>GSMTISNMEADMNRLLKQREELTKRREKLSKRREKIVKENGEGDKNVANINEEMESLTANIDY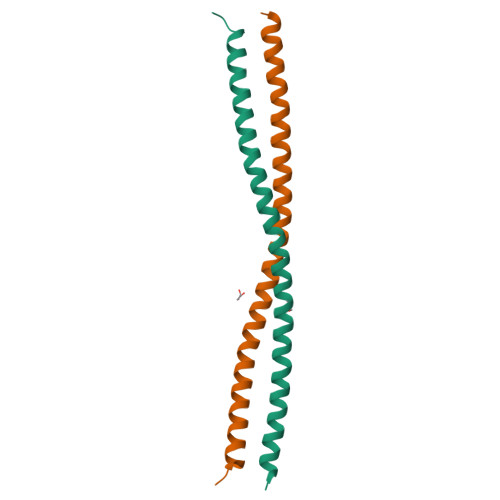INDSISDCQANIMQMEEAK[2x]>DEQPEPRTRRRAYLWCKEFLPGAWRGLREDEFHISVIRGGLSNMLFQCSLPDTTATLGDEPRKVLLRLYGAILQMRSCNKEGSEQAQKENEFQGAEAMVLESVMFAILAERSLGPKLYGIFPQGRLEQFIPSRRLDTEELSLPDISAEIAEKMATFHGMKMPFNKEPKWLFGTMEKYLKEVLRIKFTEESRIKKLHKLLSYN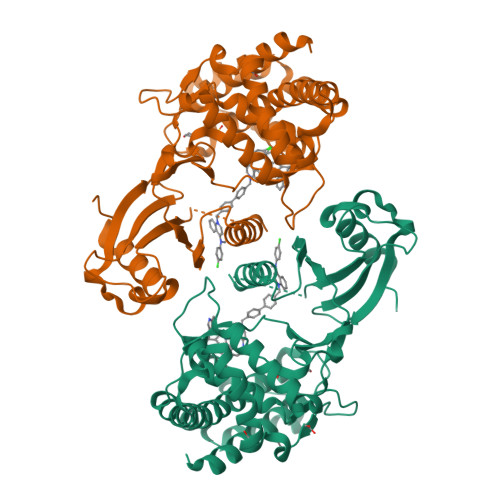LPLELENLRSLLESTPSPVVFCHNDCQEGNILLLEGRENSEKQKLMLIDFEYSSYNYRGFDIGNHFCEWMYDYSYEKYPFFRANIRKYPTKKQQLHFISSYLPAFQNDFENLSTEEKSIIKEEMLLEVNRFALASHFLWGLWSIVQAKISSIEFGYMDYAQARFDAYFHQKRKLGV[2x]Dihydropyrimidinase catalyzes the reversible cyclization of dihydrouracil to N-carbamoyl-β-alanine in the second step of the pyrimidine degradation pathway. Dihydropyrimidinase, hydantoinase, imidase, allantoinase, and dihydroorotase belong to the cyclic amidohydrolase family because of their functional and structural similarities. Most of the active sites of dihydropyrimidinases, hydantoinases, allantoinases, and dihydroorotases contain four histidines, one aspartate, and one carboxylated lysine residue, which are required for metal binding and catalytic activity. The global architecture of the dihydropyrimidinase monomer consists of two domains, namely, a large domain with a classic (β/α)8-barrel structure core embedding the catalytic dimetal center and a small β-sandwich domain.

To confirm this result and determine how this enzyme can also form a tetramer, we also determined the crystal structure of P. aeruginosa PAO1 dihydropyrimidinase at 2.17 Å resolution at acidic environment. Crystals of P. aeruginosa dihydropyrimidinase were grown at room temperature by hanging drop vapor diffusion in 10% PEG 8000, 100 mM HEPES, 200 mM calcium acetate, pH 5.9. The crystals of P. aeruginosa dihydropyrimidinase grown under this condition belonged to space group C2221 with cell dimensions of a = 108.9, b = 155.7, and c = 235.6 Å. An asymmetric unit of the crystal contained four crystallographically independent P. aeruginosa dihydropyrimidinase monomers, in which two zinc ions were found in the active site per monomer. Thus, P. aeruginosa dihydropyrimidinase did exist as a mixture of dimers and tetramers at pH 5.9. In the crystal of P. aeruginosa dihydropyrimidinase, the four molecules formed two pairs of dimers, B-A and C-D, respectively. We noted that in the crystal, another crystallographically related tetramer B-A-C′-D′ was formed and further stabilized via many hydrogen bonds and salt bridges. For the tetramer formation of P. aeruginosa dihydropyrimidinase, many hydrogen bonds with close distance were found: these bonds (<3 Å) include K374(A)–E14(B), H13(A)–E14(B), R386(A)–E14(B), R386(A)–E15(B), R467(A)–V354(B), R468(A)–G357(B), E14(A)–H13(B), E15(A)–R386(B), V354(A)–R467(B), G357(A)–R468(B), H13(C′)–E14(D′), R386(C′)–E15(D′), R468(C′)–G357(D′), E14(C′)–H13(D′), E14(C′)–K374(D′), E15(C′)–R386(D′), and G357(C′)–R468(D′); however, these residues were not found for the tetramer formation of Thermus sp. dihydropyrimidinase. Comparison by superimposition indicated that many Arg residues (R253, R358, R386, R467, and R468) found in P. aeruginosa dihydropyrimidinase, but not in Thermus sp. dihydropyrimidinase, may play a crucial role for the pH-dependent oligomerization. On the basis of these results, we concluded that P. aeruginosa dihydropyrimidinase could form a tetramer, but its oligomerization mechanism differed from those of other dihydropyrimidinases such as Thermus sp. dihydropyrimidinase.

>MSLLIRGATVVTHEESYRADVLCANGLIQAIGENLETPSGCDVLDGGGQYLMPGGIDPHTHMQLPFMGTVASEDFFSGTAAGLAGGTTSIIDFVIPNPRQSLLEAFHTWRGWAQKSAADYGFHVAITWWSDEVAREMGELVAQHGVNSFKHFMAYKNAIMAADDTLVASFERCLELGAVPTVHAENGELVFHLQQKLLAQGLTGPEAHPLSRPPQVEGEAASRAIRIAETLGTPLYLVHISSREALDEIAYARAKGQPVYGEVLAGHLLLDDSVYRHPDWATAAGYVMSPPFRPVEHQEALWRGLQSGNLHTTATDHCCFCAEQKAMGRDDFSKIPNGTAGIEDRMALLWDAGVNSGRLSMHEFVALTSTNTAKIFNLFPRKGAIRVGADADLVLWDPQGSRTLSAATHHQRVDFNIFEGRTVRGIPSHTISQGKLLWAAGDLRAEPGAGRYVERPAYPSVYEVLGRRAERQRPVAVER[4x]> QFAKPEDAVKYRQSAATLMASHFGRMTPVVKGQAPYDAAQIKANVEVLKTLSALPWAAFGPGT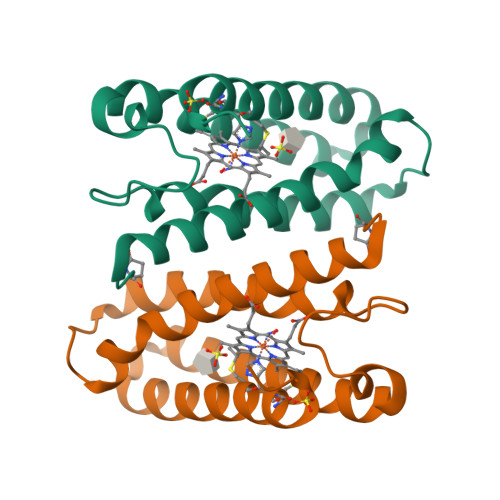EGGDARPEIWSDAASFKQKQQAFQDNIVKLSAAADAGDLDKLRAAFGDVGASCKACHDAYRKKK> GPVDPKMLRWPLRFVIGSSDTQRSLLGRIGIGDVLLIRTSRAEVYCYAKKLGHFNRV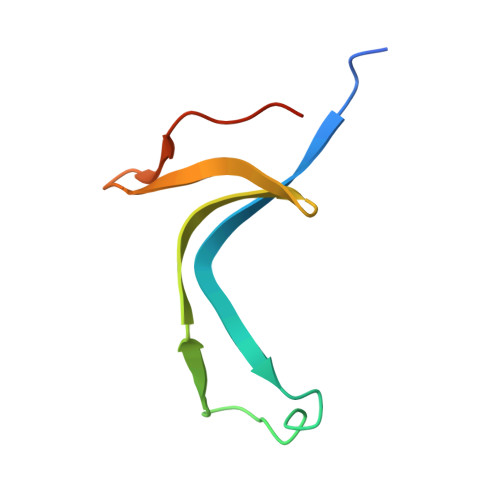EGGIIVETLDIQHIEE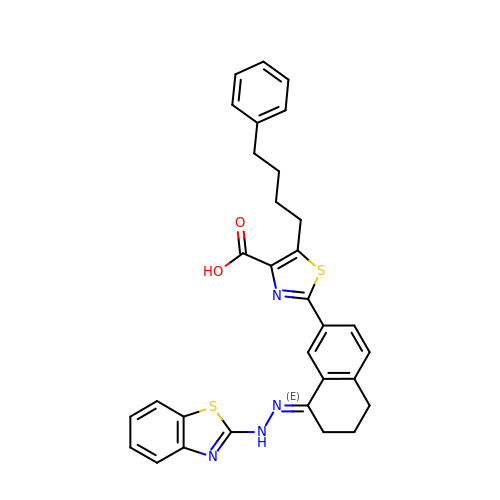2-[(8E)-8-(1,3-benzothiazol-2-ylhydrazinylidene)-6,7-dihydro-5H-naphthalen-2-yl]-5-(4-phenylbutyl)-1,3-thiazole-4-carboxylic acid | C31 H28 N4 O2 S2 | KJRCRYVHSPWAIC-JGRMKTMXSA-N(2R,3S,4S)-5-[(4R)-6',7'-dimethyl-2,3',5-trioxo-1'H-spiro[imidazolidine-4,2'-quinoxalin]-4'(3'H)-yl]-2,3,4-trihydroxypentyl-adenosine 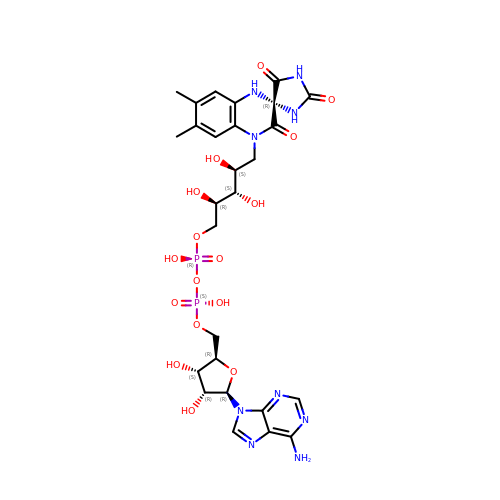diphosphate | C27 H35 N9 O16 P2 | HUPQKJNMCVRMPP-QUWWARRSSA-N> DYKDDDDAMKSILDGLADTTFRTITTDLLYVGSNDIQYEDIKGDMASKLGYFPQKFPLTSFRGSPFQEKMTAGDNPQLVPADQVNITEFYNKSLSENLYFQGSFKENEENIQCGENFMDIECFMVLNPSQQLAIAVLSLTLGTFTVLENLLVLCVILHSRSLRCRPSYHFIGSLAVADLLGSVIFVYSFIDFHVFHRKDSRNVFLFKLGGVTASFTASVGSLFLTAIDRYISIHRPLAYKRIVTRPKAVVAFCLMWTIAIVIAVLPLLGWNCEKLQSVCSDIFPHIDETYLMFWIGVTSVLLLFIVYAYMYILWKAHSHAVRMIQRGTQKSIIIHTSEDGKVQVTRPDQARMDIRLAKTLVLILVVLIICWGPLLAIMVYDVFGKMNKLIKTVFAFCSMLCLLNSTVNPIIYALRSKDLRHAFRSMFPSCEGTAQPLDNSMGDSDCLHKHANNAASVHR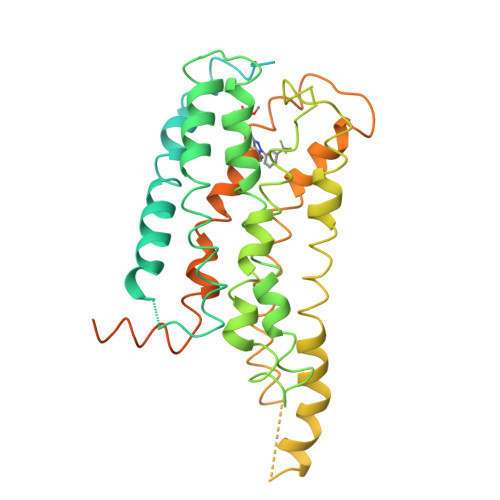AAESCIKSTVKIAKVTMSVSTDTSAEALGSHHHHHH>[2x]MTLHSWLDRYEKILASRGIKQKTLINYMSKIKAIRRGLPDAPLEDITTKEIAAMLNGYIDEGKAASAKLIRSTLSDAFREAIAEGHITTNHVAATRAAKSKVRRSRLTADEYLKIYQAAESSPCWLRLAMELAVVTGQRVGDLCEMKWSDIVDGYLYVEQSKTGVKIAIPTALHIDALGISMKETLDKCKEILGGETIIASTRREPLSSGTVSRYFMRARKASGLSFEGDPPTFHEL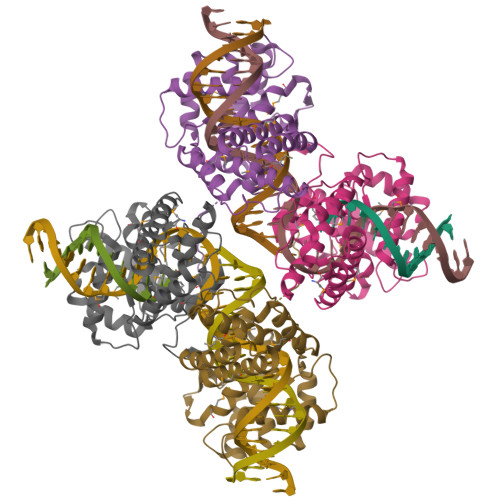RSLSARLYEKQISDKFAQHLLGHKSDTMASQYRDDRGREWDKIEIK> GHMQLSHRPAETGDLETVAGFPQDRDELFYCYPKAIWPFSVAQLAAAIAERRGSTVAVHDGQVLGFANFYQWQHGDFCALGNMMVAPAARGLGVARYLIGVMENLAREQYKARLMKISCFNANAAGLLLYTQLGYQPRAIAERHDPD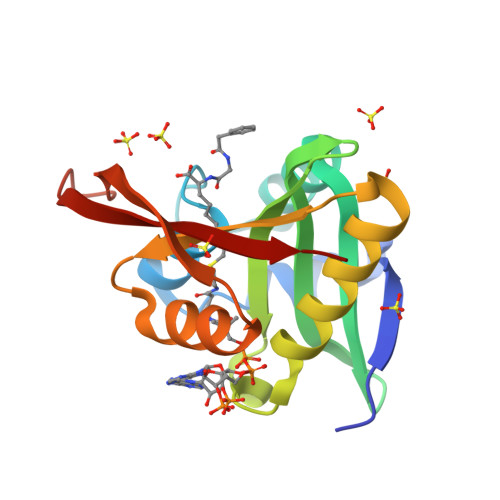GRRVALIQMDKPLE> MSEFNEKPEKLIVDGLRLDGRKFDELRPIKIEASVLKRADGSCYLEMGKNKVIAAVFGPREVHPEHLQDPS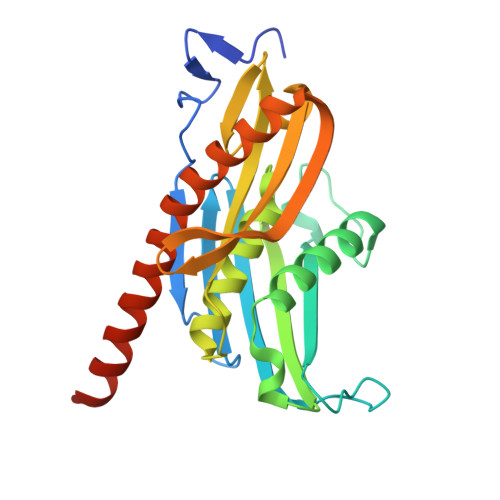KAIIRYRYNMAPFSVEERKRPGPDRRSIEISKVSKEAFEAVIMKELFPRSAIDIFVEVLQADAGSRTACLNAASVALVDAGVPMKGMITSVAVGKADGQLVLDPMKEEDNFGEADMPFAFLIRNGKIESIALLQMDGRMTRDEVKQAIELAKKGALQIYEMQREAILRRYIEVGEEMDEITEGGEDA> MGCASRDDWRCARSMHEFSAKDIDGHMVCLDKYRGFVCIVTNVA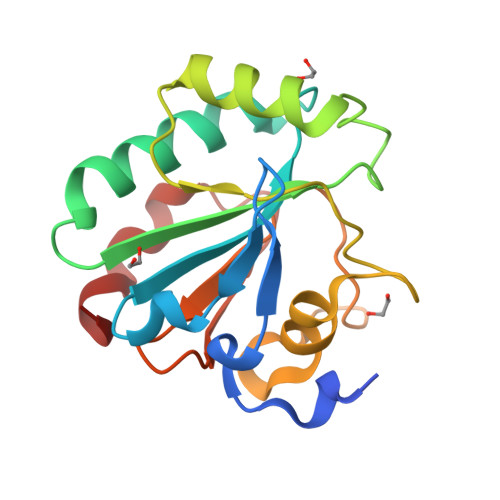SQCGKTDVNYTQLVDLHARYAECGLRILAFPCNQFGRQEPGSNQEIKEFAAGYNVKFDMYSKICVNGDDAHPLWKWMKVQPKGRGMLGNAIKWNFTKFLIDKNGCVVKRYGPMEEPQVIEKDLPCYL> FMVSLPRMVYPQPKVLTPCRKDVLVVTPWLAPIVWEGTFNIDILNEQFRLQNTTIGLTVFAIKKYVAFLKLFLETAEKHFMVGHRVHYYVFTDQPAAVPRVTLGTGRQLSVLEVGAYKRWQDVSMRRMEMISDFCER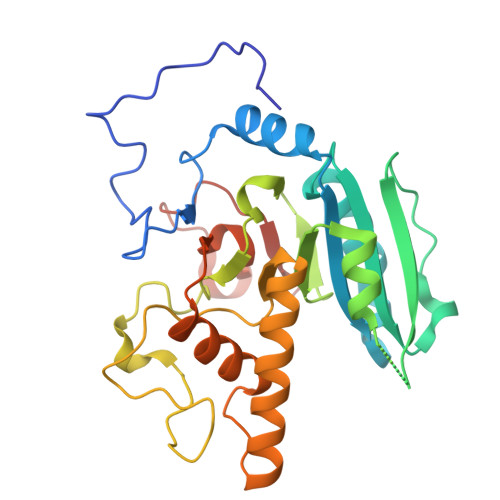RFLSEVDYLVCVDVDMEFRDHVGVEILTPLFGTLHPSFYGSSREAFTYERRPQSQAYIPKDEGDFYYMGAFFGGSVQEVQRLTRACHQAMMVDQANGIEAVWHAESHLNKYLLRHKPTKVLSPEYLWDQQLLGWPAVLRKLRFTAVPKNHQAVRNPE>[2x]IVGGRRARPHAWPFMVSLQLRGGHFCGATLIAPNFVMSAAHCVANVNVRAVRVVLGAHNLSRREPTRQVFAVQRIFENGYDPVNLLNDIVILQLNGSATINANVQVA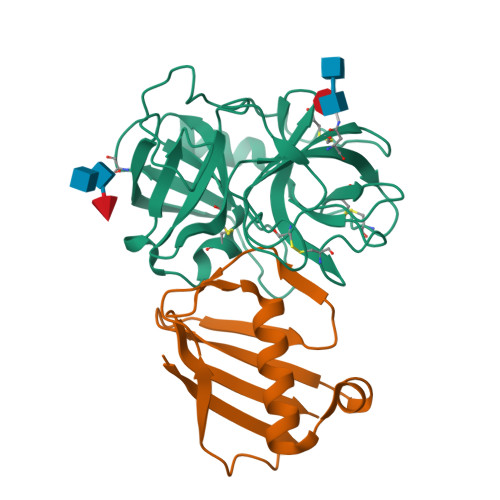QLPAQGRRLGNGVQCLAMGWGLLGRNRGIASVLQELNVTVVTSLCRRSNVCTLVRGRQAGVCFGDSGSPLVCNGLIHGIASFVRGGCASGLYPDAFAPVAQFVNWIDSIIQ;>[2x]GSTVQVPYTITVNGTSQNILSNLTFNKNQNISYKDLEGKVKSVLESNRGITDVDLRLSKQAKYTVNFKNGTKKVIDLKSGIYTANLINSSDIKSININVD>[2x]GAMELGSLCQGDSMQGQLKLGCIPTIAP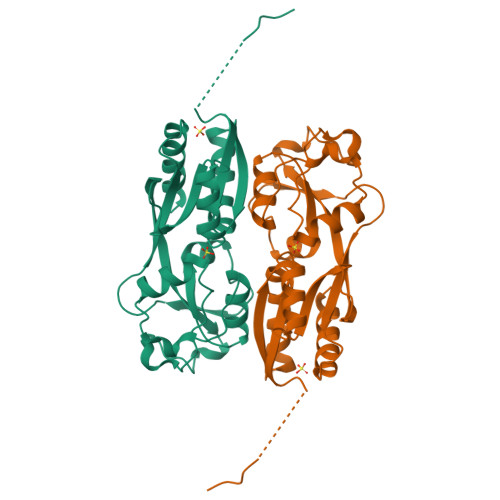FLLCDLVQEINQRFPQLNLLLREDTTTNLLTALRHGELDVLILALPVEIDGMESRVVGQDPFKMVISRHQAGAIKVPIKYDDLPDESVFLLEKEHSLTEHAVSACKLTDKEKINPFSATSLHTLVQMVANGLGTTFIPQMAIDHGLLDNQNLVVIEPPGQQAYRDIGLVWRPSSSRSKTFNQLAEVVSELL>MNFPPIGPTRVLQPYSIVNLPPLIIGGAVLNDIYTEDPTKLPIQDILSIAFSKGLNAIDTSPYYGRSEELIGKALKAITAEWPRERYYICTKAGRITDTKFDYSREHVRESVKNSLRLL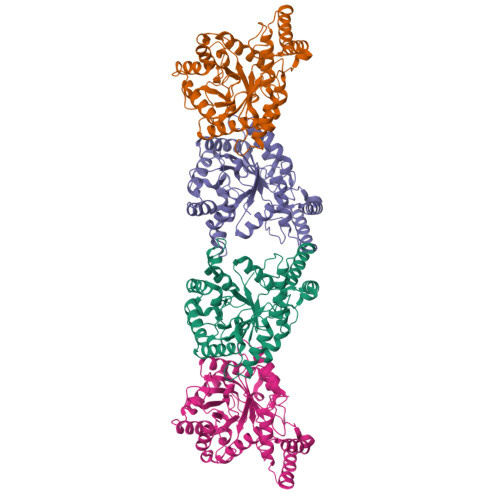NTDYLDLVYMHDVEFVETPEVYDALRELRLMKEEGLIKAFGFSGYPVKLLYEIAYKCAHDYVEDIGRVDAILSYSHGCIQNTALFELYDDFINKCGIKKILNGSILSMSLLRSGKTHAFHPASVELKAKVDEVAQDLKKTSNIELAEPATRFAMKRWLFQTQPQKDPPLKWNQRTSIVLGVSTVEELNSALKSYADVKEKDGAEDEKLFEEIIKKLGSHFNETWPSGLYSAT[4x]> FNGMELLSPKPLCSVVNCEDLEKLDHVSALNELRREQEIFKLLPGIYAHRYDFRRVSPSIINDFEYCPRLLWVQHKLGLKLLSEKSVVSIIRGRILHERYERLLSQYENVVAEYKVEIGDLVGVVDLVIKRGGEYIPVEIKTGFSKEAHKTQLQIYIS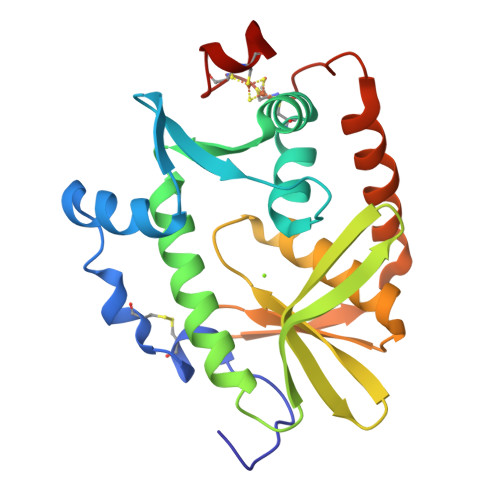MLKARFGYLVYRNHVEVVHRNDAALDVLKKIREILSAREAPPAKCNSCIFKPICKNLL> ASPDDNFSPETLQFLRNNTGLDGEQWNNIMKLINKPEQDDLNWIKYYGYCEDIEDER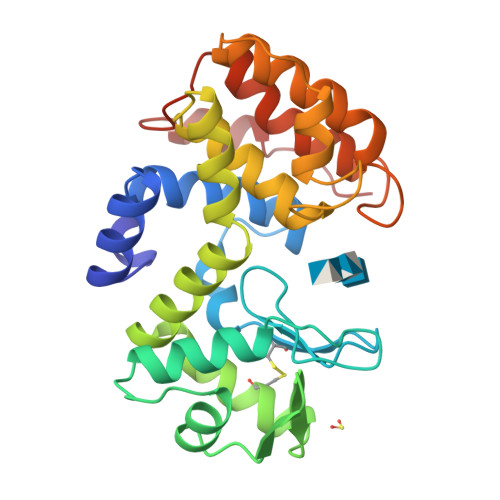GYTIGLFGATTGGSRDTHPDGPDLFKAYDAAKGASNPSADGALKRLGINGKMKGSILEIKDSEKVFCGKIKKLQNDAAWRKAMWETFYNVYIRYSVEQARQRGFTSAVTIGSFVDTALNQGATGGSDTLQGLLARSGSSSNEKTFMKNFHAKRTLVVDTNKYNKPPNGKNRVKQWDTLVDMGKMNLKNVDSEIAQVTDWEMK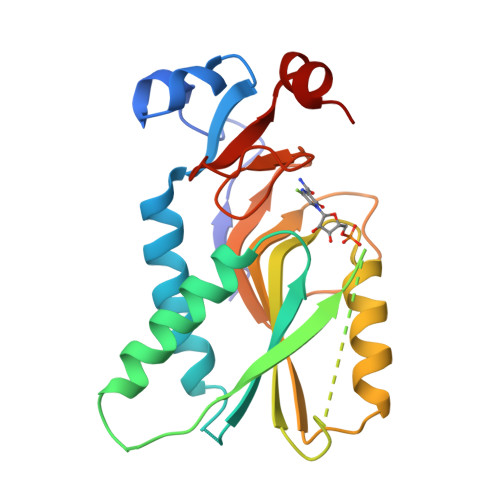> TRSPGVVISDDEPGYDLDLFCIPNHYAEDLERVFIPHGLIMDRTERLARDVMKEMGGHHIVALCVLKGGYKFFADLLDYIKALNRNSDRSIPMTVDFIRLKSYCNDQSTGDIKVIGGDDLSTLTGKNVLIVEDIIDTGKTMQTLLSLVRQYNPKMVKVASLLVKRTPRSVGYKPDFVGFEIPDKFVVGYALDYNEYFRDLNHVCVISETGKAKYKA ethyl 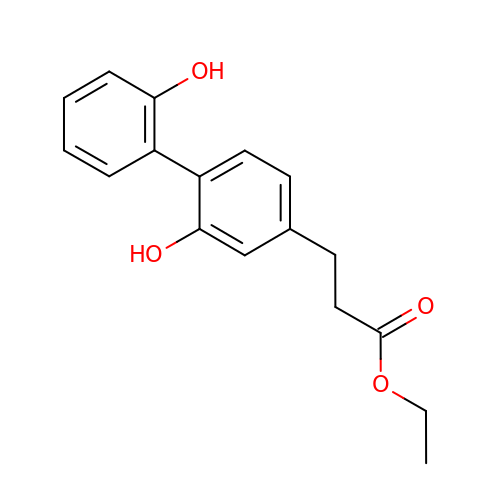3-[4-(2-hydroxyphenyl)-3-oxidanyl-phenyl]propanoate | C17 H18 O4 | NLRSDRXKCXNRRG-UHFFFAOYSA-N The point centromere of budding yeast specifies assembly of the large kinetochore complex to mediate chromatid segregation. Kinetochores comprise the centromere-associated inner kinetochore (CCAN) complex and the microtubule-binding outer kinetochore KNL1-MIS12-NDC80 (KMN) network. The budding yeast inner kinetochore also contains the DNA binding centromere-binding factor 1 (CBF1) and CBF3 complexes. The inner kinetochore centromere-associated inner kinetochore (CCAN) complex (14 to 16 subunits) associates with the centromere, generally through specific recognition of CENP-ANuc.

Previous studies identified an interaction between the essential N-terminal domain (END) of budding yeast CENP-A (CENP-AEND; residues 28 to 60) and the essential S. cerevisiae CCAN proteins CENP-Q and CENP-U. Reconstitution studies further showed that a CENP-QU module can transmit force from the outer kinetochore to CENP-ANuc. We also present a structural explanation for how the CENP-A N terminus (CENP-AN) interacts with CENP-QU. Unexpectedly, the CENP-AN binding site on CENP-QU is autoinhibited in the context of the assembled CCAN. Paradoxically, in the context of CCAN, the CENP-QUFoot is sterically blocked by an N-terminal domain of the Nkp1-Nkp2 dimer. (B) Cryo-EM map of the CENP-AN:CENP-OPQU+ (COMA) complex. In this structure, the CENP-QUFoot and adjacent coiled coil, including the CENP-AEND binding site of CENP-QU, are mobile and not visible in the cryo-EM map. In our structure, the N-terminal domain of Nkp1-Nkp2 is bent back, so only its middle region binds to CENP-QU. The remodeled Nkp1-Nkp2 releases the coiled-coil domain of CENP-QU, rendering CENP-QUFoot accessible to bind CENP-AEND. Although the CENP-QUFoot is not visible in the cryo-EM map due to conformational heterogeneity, this structure, together with the AlphaFold2 prediction, explains how CENP-AEND can bind CENP-QU in the context of Nkp1-Nkp2 and in the absence of CENP-LN. The CENP-AEND–bound CENP-QU could represent a CCAN-independent axis of inner-outer kinetochore assembly.

> MSRIDDLQQDIESLLSEINSLEESREKLKAKIKDKRKNEESANPIVQEFEDLFDQFPQLNNFLFNEHPELEETDDKDISRAQADIPATPIPYEPKKRAKLENEEILPEQEWVLKTQPMVQHQMFDPGVADLLDTDILTSPSKRKRKLKIDDISTSDRSELEDYIVLENVYRMFGITFFPLVDPIDLKIKDASGEIFVDREMLGIRLEVFSERTSQFEKPHYVLLKKRIKSNSWFLFKHTIPSFIDVQGIFDDTNGGLVISHDDAYLFAKRVFLQLVEVQKRRQIFKDLEAKKIIHDLDLDLESSMVSFFVKDIKVELFVKQNEIVSCSILDDIHDFSQNNKSKWEIALLGSLDDLELKLNHSFATIFK;> MDFTSDTTNSHDTSNSHLSLEDAVGTHHAGEADVNIDGDEKQQLSLLDDDQVRALKLQEEKDALLTRRNTLLQEIQTYQNILMKENNSKTKNGDILQNDITQDFLNLISISSSNPNSAISDRKRVERINGLTNLQKELVTKYDTLPLLNMNLRLSYLRDHTYPHLQVSVQSRDRVHNDGIEVLVVNYKFCRNTMNPFEIQFKMFYKFEDSTLLKWEILRISTNVRLKAKQLLATRNFQKCLLSLYEFDKIKSKKTGIFQNLINLLKRKTRCYLMNNSDSLIVERVIREGRLTTIKLQINFIITMPGERGKPRNCFLPMSKISIALWKGGERFNQIDLDEICYGLIKEYGVKTGLKEICNVCLFPDMYAR;> MAADRDNFLQNIENDSINNGQAMDLSPNRSSSESDSSILMNVNDIKTLRLDVAPEAKSTQSKKSLFYENSDDAEEGEIEERTNKEEGQYHHKGSKQLRFEVGKESTGKLQSHLSDGSATSGEGNVRPWEFRKVIQAEYRERLPRNYELKHWKKPSKIMIGSILRLLETNTVSALDSVFEKYEKEMNQMTHGDNNEVKRIYSKKERLLEIILTKIKKKLRQAKFPSRISERDLDIEYIYSKRQFIQNRYSQELQNNERLEAILSREQNLLEETRKLCMNLKTNNKKRLTEKLIQKDLHPVLNKAMEYTYGLESTNGFMHPDGPVTFRNDSHELNLMLNDPIKSTADVRLDKEEVLSLLPSLKEYTKKSKELKETMGQMISDSHEEEIKEVFVPHHESHQDKTEEDIH;> MDRDTKLAFRLRGSHSRRTDDIDDDVIVFKTPNAVYREENSPIQSPVQPILSSPKLANSFEFPITTNNVNAQDRHEHGYQPLDAEDYPMIDSENKSLISESPQNVRNDEDLTTRYNFDDIPIRQLSSSITSVTTIDVLSSLFINLFENDLIPQALKDFNKSDDDQFRKLLYKLDLRLFQTISDQMTRDLKDILDINVSNNELCYQLKQVLARKEDLNQQIISVRNEIQELKAGKDWHDLQNEQAKLNDKVKLNKRLNDLTSTLLGKYEGDRKIMSQDSEDDSIRDDSNILDIAHFVDLMDPYNGLLKKINKINENLSNELQPSL;> MTDTYNSISNFIENELTALLSSDDYLMDDLAGELPNEVCRLLKAQVIEKRKDAMSRGKQDLLSKEIYDNESELRASQSQQIMELVGDIPKYSLGSELRNRVEGEPQSTSIERLIEDVLKLPQMEVADEEEVEVENDLKVLSEYSNLRKDLILKCQALQIGESKLSDILSQTNSINSLTTSIKEASEDDDISEYFATYNGKLVVALEEMKLLLEEAVKTFGNSPEKREKIKKILSELKK;> MNSEQLLHNYVSDSLLTTLISFQEFKQQLQSYTSDEQQLQHWYELLQARDARVTSELEARIKQFFITLRSRLLRFLESEQLSHSLSLETLIDALYKINDLLQQRLQILDDAIQEKTSELAEFENMVRSPSAGDNAIPGLLQIIQSYINLLEEN>MGSMLILKGTKTVDLSKDELTEIIGQFDRVHIDLGTGDGRNIYKLAINDQNTFYIGIDPVKENLFDISKKIIKKPSKGGLSNVVFVIAAAESLPFELKNIADSISILFPWGTLLEYVIKPNRDILSNVADLAKKEAHFEFVTTYSDSYEEAEIKKRGLPLLS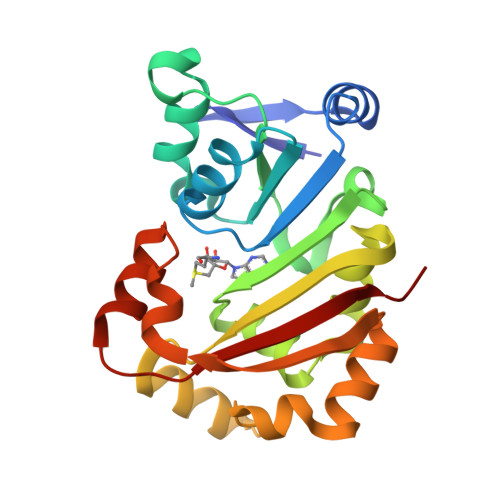KAYFLSEQYKAELSNSGFRIDDVKELDNEYVKQFNSLWAKRLAFGRKRSFFRVSGHVSKH[2x]>SGLVPRGSHMQKDFWLSEIGDKNISLGYYDDNVAIVLTNKTDKILRVYSYEDGKIRKDFEQKEIITGLMGDKKIEGDLKTPVGFYELGRKFNPGDPYYGPFA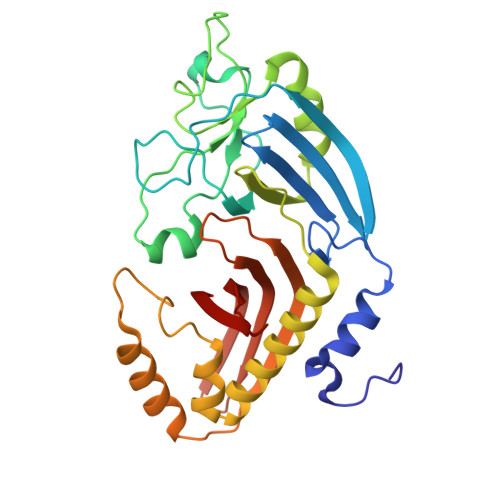FATTYPNLLDKVQGKTGGGIWIHGYPLDGSRLDEFKTRGCIALFNNNLEKFAQVVQDKKVFVMTEEKEKIRAKKDQIASLLADLFTWKLAWTNSDTNTYLSFYDEQEFKRFDKMKFEQFASMKKSIFSRKEDKKIKFSDINISPYPNLENETMYRISFYEDYYTKNYQFRGDAILYVKIDSKGKMKILAEQ[2x]2-oxidanyl-N-[[(3R)-3-oxidanyl-1-(7H-pyrrolo[2,3-d]pyrimidin-4-yl)piperidin-3-yl]methyl]-4-[[(3S)-3-propan-2-yl-2-azaspiro[3.3]heptan-2-yl]methyl]benzamide | C29 H38 N6 O3 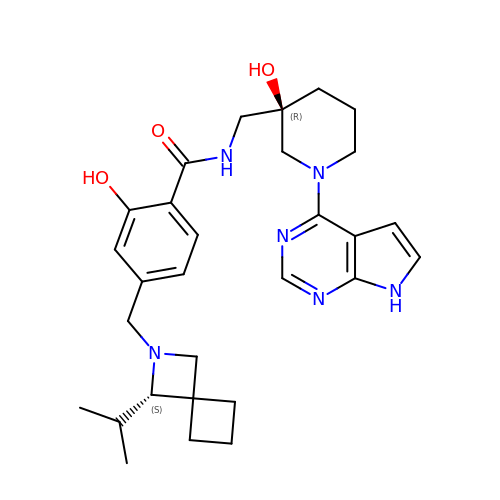| KWHHOOQYPVRBOP-PWUYWRBVSA-N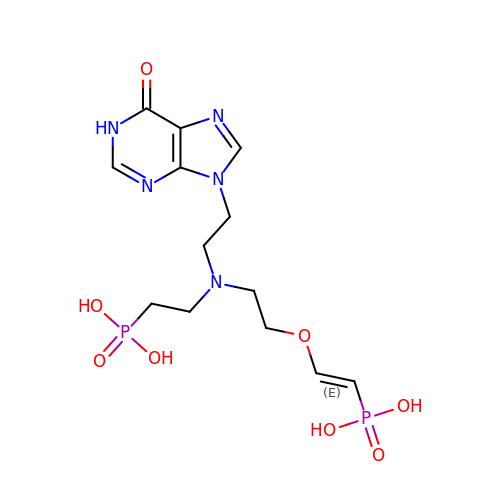(2-{[2-(6-oxo-1,6-dihydro-9H-purin-9-yl)ethyl](2-{[(E)-2-phosphonoethenyl]oxy}ethyl)amino}ethyl)phosphonic acid | C13 H21 N5 O8 P2 | SGNFOZIWXPTVIN-SOFGYWHQSA-N> ETGASYITPYVPMPCMINDTHFLLRGPFEASWAIKLEITDVTTLVVDTDNVANPTNISKCFANNQDERLLGFTMEWFLSGLEHDHHFTPQIICGNVSKGEVNAQVNITMEDHCSQVFLKMRRIFGVFKNPCTSHGKQNVLIS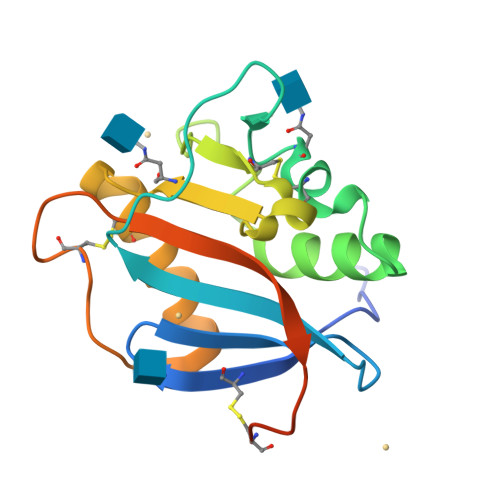VSNWTNQCSGNHLSGTKHHHHHH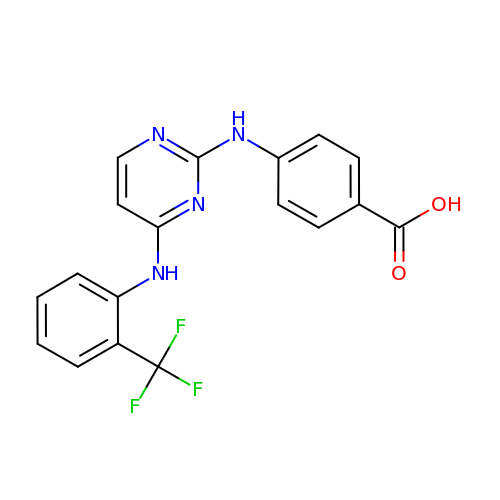4-[(4-{[2-(trifluoromethyl)phenyl]amino}pyrimidin-2-yl)amino]benzoic acid | C18 H13 F3 N4 O2 | QFNWNXOHCUAEBM-UHFFFAOYSA-N>MSALLILALVGAAVADYKDDDDKLCRLCPWDWTFLLGNCYFFSKSQRNWNDAVTACKEVKAQLVIINSDEEQTFLQQTSKAKGPTWMGLSDLKKEATWLWVDGSTLSSRFQKYWNRGEPNNIGEEDCVEFAGDGWNDSKCEL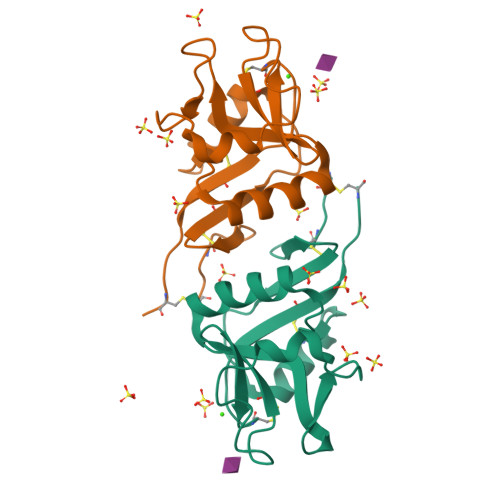KKFWICKKSATPCTEG[4x]methyl {3-[(2R)-1-{(2R)-2-(3,4-dimethoxyphenyl)-2-[(1-oxo-1,2,3,4-tetrahydroisoquinolin-7-yl)amino]acetyl}pyrrolidin-2-yl]-4-(propan-2-ylsulfonyl)phenyl}carbamate | C34 H40 N4 O8 S | 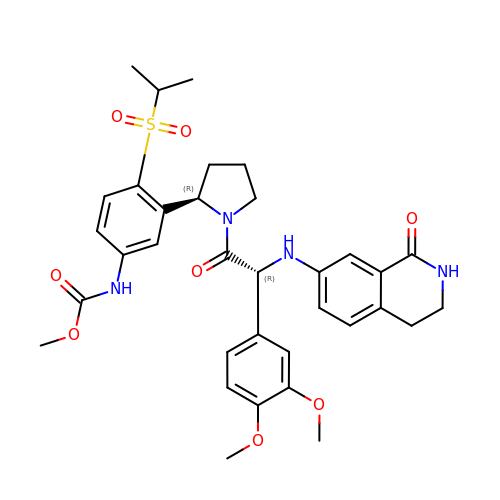XGQHTIIEXCNFSG-DLFZDVPBSA-N> GSVLTAIDNDKVAVGDKVTLTINVDKITNFSGYQFNIKYNTTYLQPWDTIADEAYTDSTMPDYGTLLQGRFNATDMSKHNLSQGVLN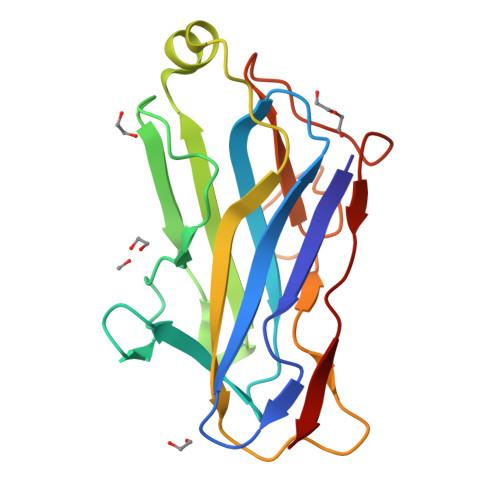FGRLYMNLSAYRASGKPESTGAVAKVTFKVIKEIPAEGIKLATFENGSSMNNAVDGTMLFDWDGNMYSSSAYKVVQPGLIYPK> PFPKPTLWAEPGSVISWGSPVTIWCQGSLEAQEYRLDKEGSPEPLDRNNPLEPKNKARFSIPSMTEHHAGRYRCHYYSSAGWSEPSDPLELVMTGFYNKPTLSALPSPVVASGGNMTLRCGSQKGYHHFVLMKEGEHQ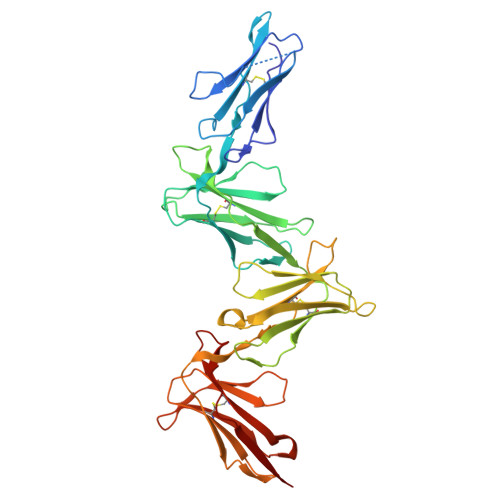LPRTLDSQQLHSGGFQALFPVGPVNPSHRWRFTCYYYYMNTPQVWSHPSDPLEILPSGVSRKPSLLTLQGPVLAPGQSLTLQCGSDVGYDRFVLYKEGERDFLQRPGQQPQAGLSQANFTLGPVSRSHGGQYRCYGAHNLSSEWSAPSDPLNILMAGQIYDTVSLSAQPGPTVASGENVTLLCQSWWQFDTFLLTKEGAAHPPLRLRSMYGAHKYQAEFPMSPVTSAHAGTYRCYGSYSSNPHLLSFPSEPLELMVSG>STAGKVIKCKAAVLWEEKKPFSIEEVEVAPPKAHEVRIKMVATGICRSDDHVVSGTLVTPLPVIAGHEAAGIVESIGEGVTTVRPGDKVIPLFTPQCGKCRVCKHPEGNFCLKNDLSMPRGTMQDGTSRFTCRGKP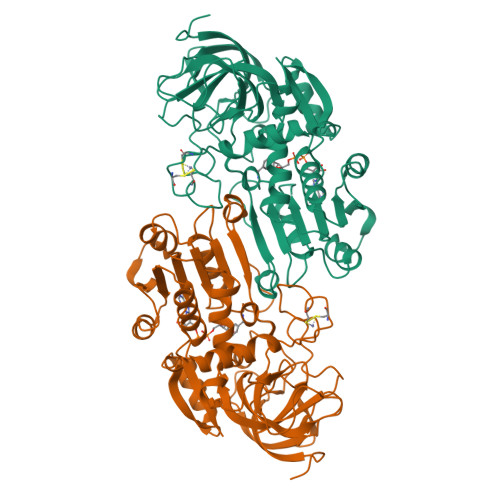IHHFLGTSTFSQYTVVDEISVAKIDAASPLEKVCLIGCGFSTGYGSAVKVAKVTQGSTCAVFGLGGVGLSVIMGCKAAGAARIIGVDINKDKFAKAKEVGATECVNPQDYKKPIQEVLTEMSNGGVDFSFEVIGRLDTMVTALSCCQEAYGVSVIVGVPPDSQNLSMNPMLLLSGRTWKGAIFGGFKSKDSVPKLVADFMAKKFALDPLITHVLPFEKINEGFDLLRSGESIRTILTF[2x]In mammals, DNA methylation is stably propagated by DNA methyltransferase 1 (DNMT1) during mitotic division. DNMT1 contains a C-terminal methyltransferase (MTase) domain, preceded by several regulatory domains including a replication-foci-targeting sequence (RFTS), a CXXC zinc finger domain and a pair of bromo-adjacent homology (BAH) domains. Here, we report that DNA methyltransferase 1 (DNMT1) specifically ‘recognizes’ H4K20me3 via its first bromo-adjacent-homology domain (DNMT1BAH1). Here, we show that DNMT1 directly recognizes H4K20me3 through the regulatory domain BAH1, which in turn mediates the chromatin association and enzymatic activation of DNMT1.

To elucidate the H4K20me3-binding specificity, we also determined the crystal structure of bDNMT1BAH1 in complex with the H414–25K20me2 peptide at 2.8 Å resolution. The structure of bDNMT1BAH1–H4K20me2 reveals a similar interaction mode as that of bDNMT1BAH1–H4K20me3, with the side chain of H4K20me2 surrounded by the same set of H4K20me3-binding residues (boxed). Distinct from the previously determined structure of the ORC1BAH–H4K20me2 complex in which the dimethylammonium group of H4K20me2 forms a hydrogen bond with a surrounding glutamate (ORC1BAH E93), the side chain of H4K20me2 in the bDNMT1BAH1 complex is not within a hydrogen-bond distance with the side-chain carboxylates of D799 and E816, thus explaining why hDNMT1BAH1 shows a relative lower binding affinity for H4K20me2 than for H4K20me3. Along the line, titration of hDNMT1BAH1 with the H414–25K20me3 and H414–25K20me2 peptides gave dissociation constants (Kd) of 2.7 and 4.1 μM, respectively, compared to the Kd values of 10.6 and 17.9 μM determined for hDNMT1BAH1 with H414-25K20me1 and H414–25K20me0, respectively. Mutation of hDNMT1BAH1 at or near the corresponding H4K20me3-binding pocket residues (D768A, Y775A, E819A, and E821A) significantly reduced its binding affinity for the H414–25K20me3 or H414–25K20me2 peptide, while introduction of a W796A mutation largely abolishes the hDNMT1BAH1–H414–25K20me3 or hDNMT1BAH1–H414–25K20me2 binding. These observations suggest that DNMT1 has evolved with a conserved mechanism for H4K20me2/3 recognition.

>SKNRISWVGDAVKTDGKKSYYKKVCIDSETLEVGDCVSVIPDDSSKPLYLARVTALWEDSSNGQMFHAHWFCAGTDTVLGATSDPLELFLVDECEDMQLSYIHSKVQVIYKAPSGAGSATYFYQLWYDQDYARFESPPKTQPTEDNKYKFCASCARLA[4x];>[4x]GAKRHRKVLRDNY>MASKKVCIVGSGNWGSAIAKIVGGNAAQLAQFDPRVTMWVFEEDIGGKKLTEIINTQHENVKYLPGHKLPPNVVAVPDVVQAAEDADILIFVV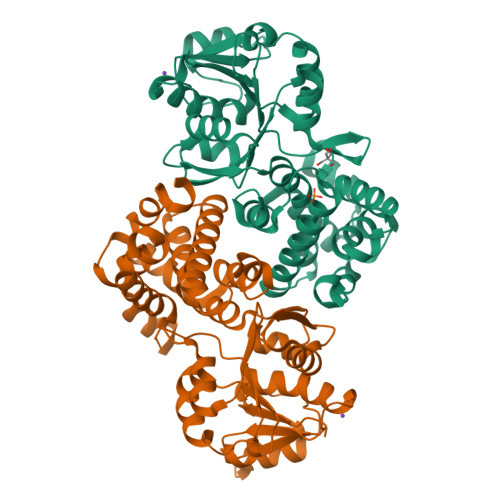PHQFIGKICDQLKGHLKANATGISLIKGVDEGPNGLKLISEVIGERLGIPMSVLMGANIASEVADEKFCETTIGCKDPAQGQLLKELMQTPNFRITVVQEVDTVEICGALKNVVAVGAGFCDGLGFGDNTKAAVIRLGLMEMIAFAKLFCSGPVSSATFLESCGVADLITTCYGGRNRKVAEAFARTGKSIEQLEKELLNGQKLQGPETARELYSILQHKGLVDKFPLFMAVYKVCYEGQPVGEFIHCLQNHPEHM[2x]> MDYKDDDDKRSPVRDLARNDGEESTDRTPLLPGAPRAEAAPVCCSARYNLAILAFFGFFIVYALRVNLAVALVDMVDSNTTLEDNRTSKACPEHSAPIKVHHNQTGKKYQWDAETQGWILGSFFYGYIITQIPGGYVASKIGGKMLLGFGILGTAVLTLFTPIAADLGVGPLIVLRALEGLGEGVTFPAMHAMWSSWAPPLERSKLLSISYAGAQLGTVISLPLSGIICYYMNWTYVFYFFGTIGIFWFLLWIWLVSDTPQKHKRISHYEKEYILSSLRNQLSSQKSVPWVPILKSLPLWAIVVAHFSYNWTFYTLLTLLPTYMKEILRFNVQENGFLSSLPYLGSWLCMILSGQAADNLRAKWNFSTLCVRRIFSLIGMIGPAVFLVAAGFIGCDYSLAVAFLTISTTLGGFCSSGFSINHLDIAPSYAGILLGITNTFATIPGMVGPVIAKSLTPDNTVGEWQTVFYIAAAINVFGAIFFTLFAKGEVQNWALNDHHGHRH

Sialin, a member of the solute carrier 17 (SLC17) transporter family, is unique in its ability to transport not only sialic acid using a pH-driven mechanism, but also transport mono and diacidic neurotransmitters, such as glutamate and N-acetylaspartylglutamate (NAAG), into synaptic vesicles via a membrane potential-driven mechanism. Sialin (SLC17A5) belongs to the solute carrier 17 (SLC17) transporter subfamily that includes nine related transmembrane major facility superfamily (MFS) transporters, all of which are dedicated to anion transport, including the vesicular glutamate transporters 1-3 (VGLUT1–3) and a vesicular nucleotide transporter (VNUT). Sialin adopts a classical MFS fold consisting of 12 transmembrane helices (TMs) with two pseudo-symmetric domains: N-domain (TMs 1-6) and C-domain (TMs 7-12). The Sialin structures in both the lumen-open and cytosol-open conformations reveal a solvent-accessible cavity, which forms the substrate translocation pathway, at the center of the interface between the N-domain and C-domain.

Moreover, we determined the cryo-EM structure of the SialinS61A in complex with Fab10B8 at 3.2-Å resolution. The structure of SialinS61A is in a lumen-open state. The interaction between Arg57 and Arg168 is disrupted, instead, Arg168 forms the salt bridge with Glu171, which is consistent with our observation on SialinR168K. These findings support our hypothesis of the hydrophilic interaction network in the luminal leaflet to modulate the conformational change of Sialin. Indeed, the S61A and R168K mutations confine Sialin in the lumen-open state, indicating the importance of these residues in regulating the conformation of Sialin. To functionally test these interactions, we mutated Ser61, Tyr306, Leu309 and Tyr335 to alanine individually. As a result, the sialic acid transport activity was considerably reduced, indicating that these residues play critical roles in the transport cycle. The lumen-open structure reveals that the hydrophilic interactions between Arg195 on TM5 and Gln273 on the cytosolic helix, Ser196 on TM5 and Arg353 on TM8, Lys197 on TM5 and Asp350 on TM8 seal the substrate translocation pathway from the cytosolic space.Cell surface layers (S-layers) form symmetrical lattices on many bacterial and archaeal cells, playing essential roles such as facilitating cell adhesion, evading the immune system, and protecting against environmental stress. The S-layer is built from one or more (glyco)-protein subunits, S-layer proteins (SLPs), that self-assemble into a highly flexible and dynamic lattice through an entropy-driven process, allowing for structural adaptation in response to changing environmental conditions. In this study, we introduce the SymProFold pipeline, which utilizes the high accuracy of AlphaFold-Multimer predictions to derive symmetrical assemblies from protein sequences, specifically focusing on two-dimensional S-layer arrays and spherical viral capsids. The predicted models were validated using available experimental data at the cellular level, and additional crystal structures were obtained to confirm the symmetry and interfaces of several SymProFold assemblies.

High-resolution experimental data confirming the proposed assemblies at the atomic level is very scarce. Based on our predicted models of Viridibacillus arvi and Methanococcus voltae, we designed constructs (see Methods section) containing only the domain responsible for the formation of either the 4-fold or 2-fold axis. G Proposed assembly of Viridibacillus arvi (gray) with the 4-fold symmetry axis shown in orange. Aligning the crystal structures with the SymProFold models revealed a great similarity, with RMSD values of 0.65 Å for V. arvi and 1.38 Å for M. voltae, further confirming our predicted assemblies. For the assembly prediction of S-layers from B. brevis and V. arvi (Slp1), an additional region above the core, responsible for the self-assembly, is present. The domains and residues in this layer might be important for interaction with the environment, including the host.

>[4x]MASAVLVTGEVSNVDLDKTTITISEDGKTFNYNYEEAIFKLHNNVVSQSKFESLLFGATVTASKDDKGVLTLNIIDEGVDALEHHHHHH> GSMEPPNLYPVKLYVYDLSKGLARRLSPIMLGKQLEGIWHTSIVVHKDEFFFGSGGISSCPPGGTLLGPPDSVVDVGSTEVTEEIFLEYLSSLGESLFRGEAYNLF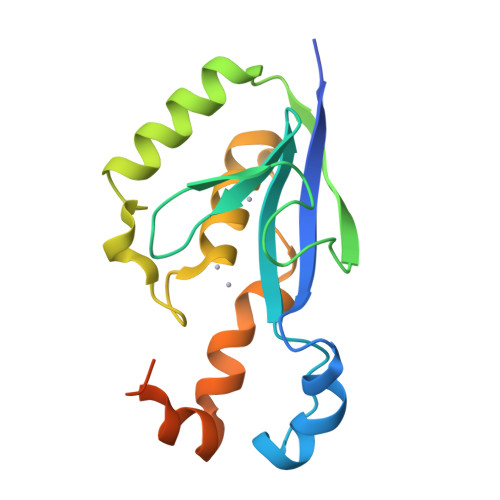EHNCNTFSNEVAQFLTGRKIPSYITDLPSEVLSTPFGQALRPLLDSIQIQPPGGSSVGRPNGQS>SRVIVHVDLDCFYAQVEMISNPELKDKPLGVQQKYLVVTCNYEARKLGVKKLMNVRDAKEKCPQLVLVNGEDLTRYREMSYKVTELLEEFSPVVERLGFDENFVDLTEMVEKRLQQLQSDELSAVTVSGHVYNNQSINLLDVLHIRLLVGSQIAAEMREAMYNQLGLTGCAGVASNKLLAKLVSGVFKPNQQTVLLPESCQHLIHSLNHIKEIPGIGYKTAKCLEALGINSVRDLQTFSPKILEKELGISVAQRIQKLSFGEDNSPVILSGPPQSFSEEDSFKKCSSEVEAKNKIEELLASLLNRVCQDGRKPHTVRLIIRRYSSEKHYGRESRQCPIPSHVIQKLGTGNYDVMTPMVD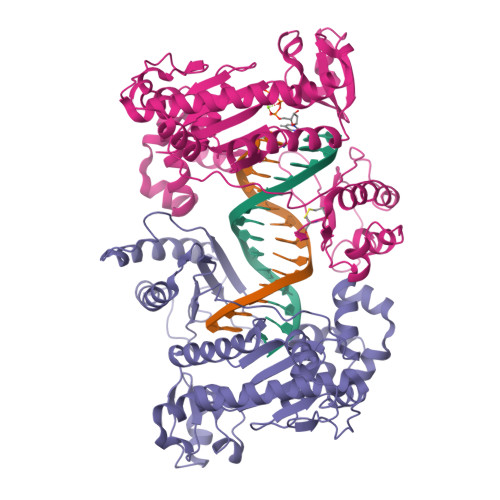ILMKLFRNMVNVKMPFHLTLLSVCFCNLK[2x]4-[(4,4-dimethylpiperidin-1-yl)methyl]-~{N}-[[(3~{S})-1-[6-(methylamino)pyrimidin-4-yl]-3-oxidanyl-piperidin-3-yl]methyl]-2-oxidanyl-benzamide | C26 H38 N6 O3 | 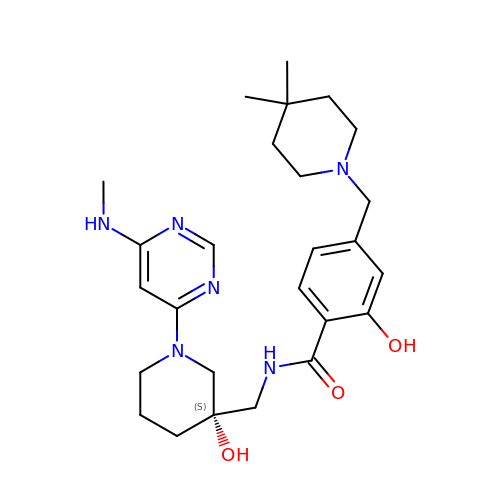BEGALFNTKBNFJE-SANMLTNESA-N> SSEDSFV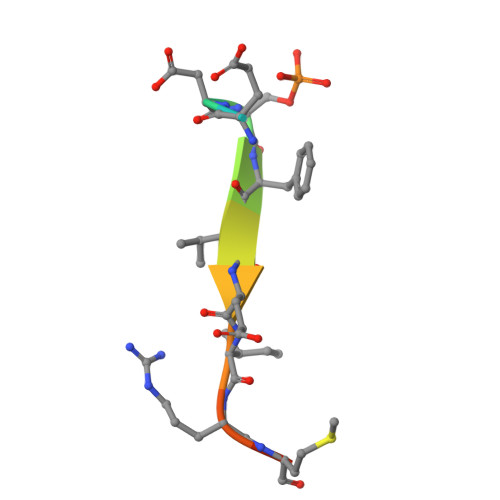EIRMAE>[4x]DWVIPPINLPENSRGPFPQELVRIRSDRDKNLSLRYS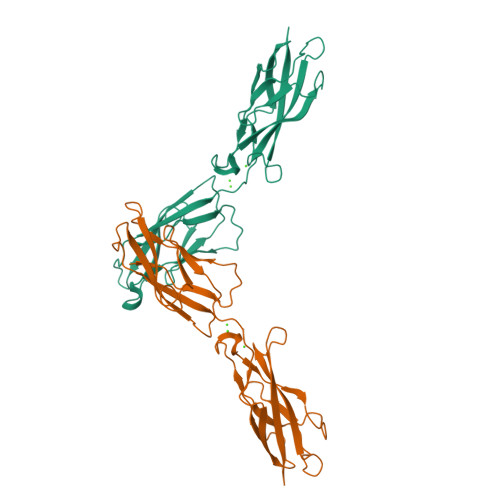VTGPGADQPPTGIFIINPISGQLSVTKPLDRELIARFHLRSHAVDINGNQVENPMDIVINVIDMNDNRPEFLHQVWNGSVPEGSKPGTYVMTVTAIDADDPNALNGMLRYRILSQAPSTPSPNMFTINNETGDIITVAAGLDREKVQQYTLIIQATDMEGNPTYGLSNTATAVITVTD>MSRFVTSVSALAMLALAPAALSSGAYANDKLVELSKSDDNWVMPGKNYDSNNFSDLKQINKGNVKQLRPAWTFSTGLLNGHEGAPLVVDGKMYIHTSFPNNTFALGLDDPGTILWQDKPKQNPAARAVACCDLVNRGLAYWPGDGKTPALILKTQLDGNVAALNAETGETVWKVENSDIKVGSTLTIAPYVVKDKVIIGSSGAELGVRGYLTAYDVKTGEQVWRAYATGPDKDLLLASDFNIKNPHYGQKGLGTGTWEGDAWKIGGGTNWGWYAYDPGTNLIYFGTGNPAPWNETMRPGDNKWTMTIFGRDADTGEAKFGYQKTPHDEWDYAGVNVMMLSEQKDKDGKARKLLTHPDRNGIVYTLDRTDGALVSANKLDDTVNVFKSVDLKTGQPVRDPEYGTRMDHLAKDICPSAMGYHNQGHDSYDPKRELFFMGINHICMDWEPFMLPYRAGQFFVGATLNMYPGPKGDRQNYEGLGQIKAYNAITGDYKWEKMERFAVWGGTMATAGDLVFYGTLDGYLKARDSDTGDLLWKFKIPSGAIGYPMTYTHKGTQYVAIYYGVGGWPGVGLVFDLADPTAGLGAVGAFKKLANYTQMGGGVVVFSLDGKGPYDDPNVGEWKSAAKHHHHHH[2x];>MSLVNGRRRTAASVVALTAALTALAALCAPAQAQDTKATSKAAEAAKPDAGTLRVCAAEQPPLSMKDGSGLENRIATTVAEAMGRKAQFVWLGKPAIY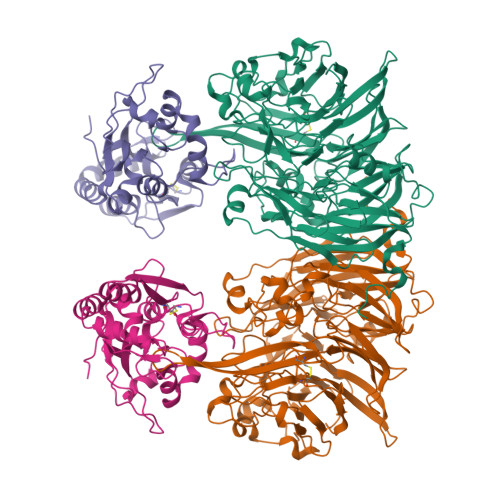LVRDGLEKKTCDVVIGLDADDPRVLTSKPYYRSGYVFLTRADKDLDIKSWSDPRLKEVSHMVVGFGTPGEAMLKDIGRYEEDMAYLYSLVNFRAPRNQYTQIDPARMVSEVATGKAEVGVAFGPDVARYVRDSSTKLRMTPVPDDTQASDGRKMPQSFDQAMGVRKDDTALKAEIDAALEKAKPKIEAILKEEGVPVLPVSN[2x]>[2x]YFQSMQKLQALKDTANRLRISSIQATTAAGSGHPTSCCSAAEIMAVLFFHTMRYKSQDPRNPHNDRFVLSKGHAAPILYAVWAEA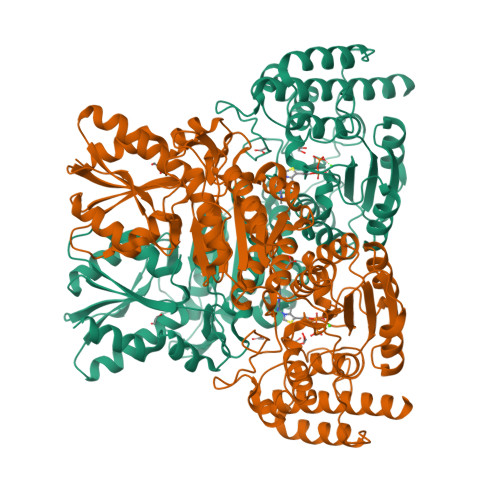GFLAEAELLNLRKISSDLDGHPVPKQAFTDVATGSLGQGLGAACGMAYTGKYFDKASYRVYCLLGDGELSEGSVWEAMAFASIYKLDNLVAILDINRLGQSDPAPLQHQMDIYQKRCEAFGWHAIIVDGHSVEELCKAFGQAKHQPTAIIAKTFKGRGITGVEDKESWHGKPLPKNMAEQIIQEIYSQIQSKKKILATPPQEDAPSVDIANIRMPSLPSYKVGDKIATRKAYGQALAKLGHASDRIIALDGDTKNSTFSEIFKKEHPDRFIECYIAEQNMVSIAVGCATRNRTVPFCSTFAAFFTRAFDQIRMAAISESNINLCGSHCGVSIGEDGPSQMALEDLAMFRSVPTSTVFYPSDGVATEKAVELAANTKGICFIRTSRPENAIIYNNNEDFQVGQAKVVLKSKDDQVTVIGAGVTLHEALAAAELLKKEKINIRVLDPFTIKPLDRKLILDSARATKGRILTVEDHYYEGGIGEAVSSAVVGEPGITVTHLAVNRVPRSGKPAELLKMFGIDRDAIAQAVRGLI> KKVYKPEVQLRRPNWSKFVAEDLSQDCFWTKVKEDRFENNELFAKLTLAFSAQTKTSKAKKDQEGGEEKKSVQKKKVKELKVLDSKTAQNLSIFLGSFRMPYQEIKNVILEVNEAVLTESMIQNLIKQMPEPEQLKMLSELKEEYDDLAESEQFGVVMGTVPRLRPRLNAILFKLQFSEQVENIKPEIVSVTAACEELRKSENFSSLLELTLLVGNYMNAGSRNAGAFGFNISFLCKLRDTKSADQKMTLLHFLAELCENDHPEVLKFPDELAHVEKASRVSAENLQKSLDQMKKQIADVERDVQNFPAATDEKDKFVEKMTSFVKDAQEQYNKLRMMHSNMETLYKELGDYFVFDPKKLS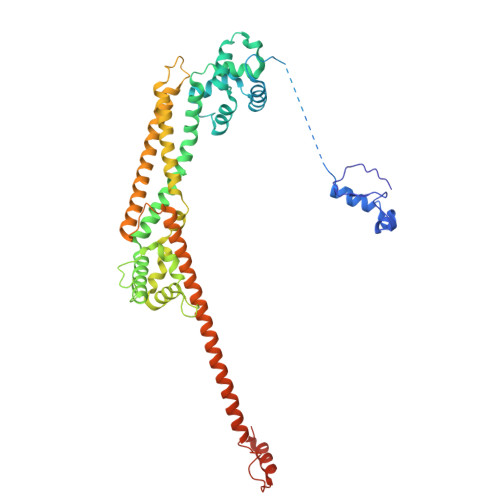VEEFFMDLHNFRNMFLQAVKENQKRRETEEKMRRAKLAKEKAEKERLEKQQKREQLIDMNAEGDETGVMDSLLEALQSGAAFRRKRGPRQVNRKAG> GHLDDNVTQEDIQAMLQEGSSAGVIEHNEHAMVKNVFRLDERTISSLMVPRSDIVFLDLNLPLDANLRTVMQSPHSRFPVCRNNVDDMVGIISAKQLLSESIAGERLELVDLVKNCNFVPNSLSGMELLEHF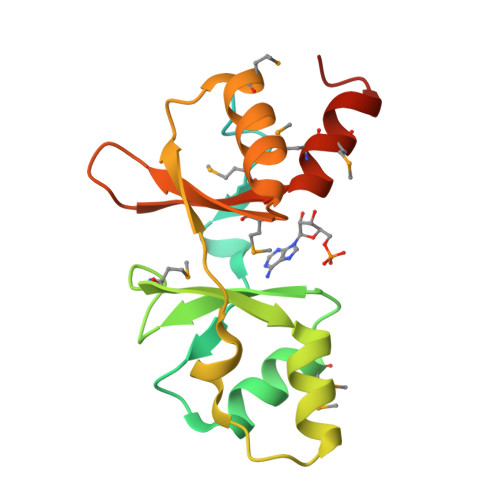RTTGSQMVFVVDEYGDLKGLVTLQDMMDALTGEFFQEDGS> GQQPVNHLVKEIDMLLKEYLLSGDISEAEHCLKELE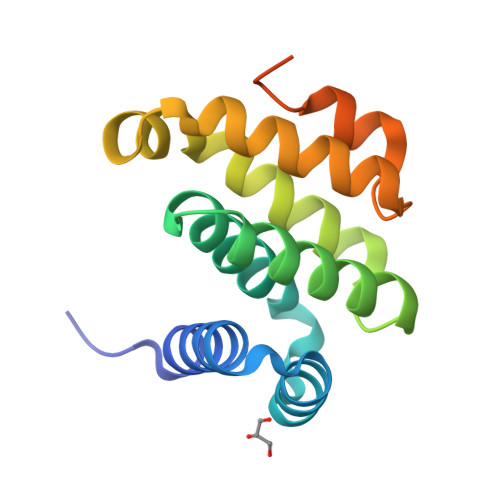VPHFHHELVYEAIVMVLESTGESAFKMILDLLKSLWKSSTITIDQMKRGYERIYNEIPDINLDVPHSYSVLERFVEECFQAGIISKQLRDLCPSRSRGRKRFVSEGDGGRLKPESY>[2x]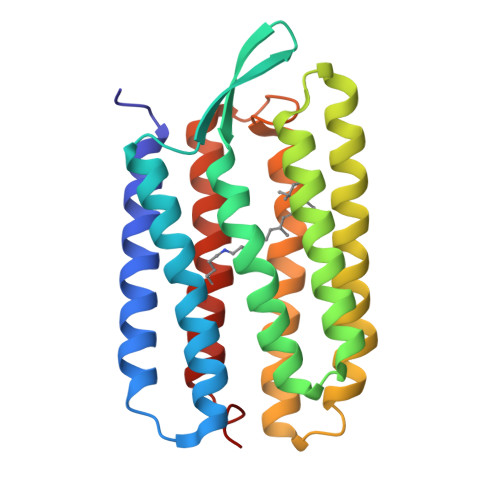TGRPEWIWLALGTALMGLGSLYFLVKGMGVSDPDAKKFYAITTLVPAIAFTMYLSMLLGYGLTMVPFGGEQNPIYWARYADWLFTTPLLLLDLALLVDADQGTILALVGADGIMIGTGLVGALTKVYSYRFVWWAISTAAMLYILYVLFFGFTSKAESMRPEVASTFKVLRNVTVVLWSAYPVVWLIGSEGAGIVPLNIETLLFMVLDVSAKVGFGLILLRSRAIFG>[7x]MNHKVHHHHHHIEGRHMTELKSKFVKVYSVLKKELLHDSAFGLTDDSRNWVERIMDYNVPGGKLNRGLSVVDSYKLLRELTNSKYKSELSDDEIFLASVLGWSVEWIQACAL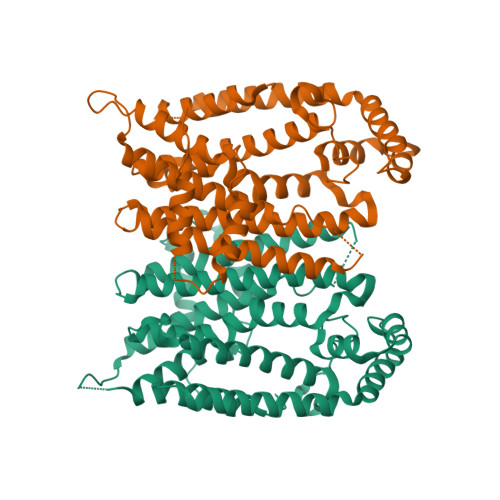VLDDIMDHSHTRRGHPCWFRLPKVGMIAINDGLILRNHVPRILRTHFQTEHYYLQLVDLFHEVECQTIAGQMLDLITTLAGEINLSSYSLPVYQQITLSKTSYYSFYLPVACALVMLGENLESHDDMKDILLEMGTYFQVQDDYLDCFGDPEVIGKIGTDIEDNKCTWLVVQALEHCNEEQKKLLYDNYGRKDPKQVAKVKELYKTLNLEDLFTQYENKTCKKLTKSIEALPNVAVQAVLKSFLAKIHKRLK>MTPNIYQQLGLKKVINACGKMTILGVSSVAPEVMQATARAASAFVEIDALVEKTGELVSRYTGAEDSYITSCASAGIAIAVAAAITHGDRARVALMPDSSGMANEVVMLRGHNVDYGAPVTSAIRLGGGRIVEVGSSNLATRWQLESAINEKTAALLYVKSHHCVQKGMLSIDDFVQVAQANHLPLIVDAAAEEDLRGWVASGADMVIYSGAKAFNAPTSGFITGRKTWIAACKAQHQGIARAMKIGKENMVGLVYALENYHQGQTTVTAAQLQPVAEAISAIHGLYADIEQDEAGRAIWRIRVRVNASELGLN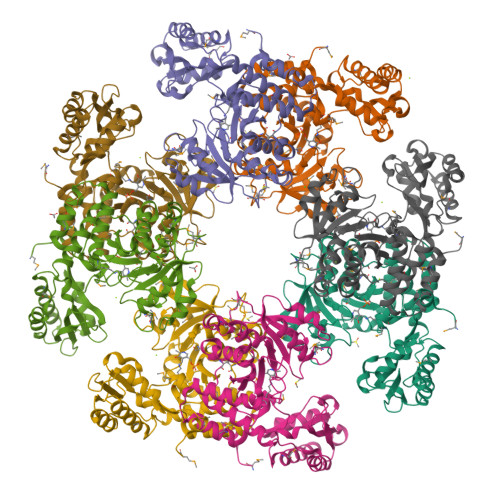AQDVEAQLRGGEIAIYARKYQLHQGVFSLDPRTVAEGEMALIVARLREIAEHAAD[8x]> MKSNEHDDCQVTNPSTGHLFDLSSLSGRAGFTAAYSEKGLVYMSICGENENCPPGVGACFGQTRISVGKANKRLRYVDQVLQLVYKDGSPCPSKSGLSYKSVISFVCRPEAGPTNRPMLISLDKQTCTLFFSWHTPLACEQATECSVRNGSSIVDLSPLIHRTGGYE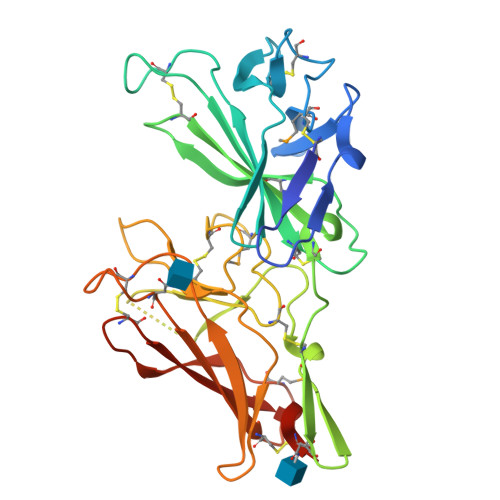AYDESEDDASDTNPDFYINICQPLNPMHAVPCPAGAAVCKVPIDGPPIDIGRVAGPPILNPIANEIYLNFESSTPCLADKHFNYTSLIAFHCKRGVSMGTPKLLRTSECDFVFEWETPVVCPDEVKHHHHHH Here, we determine mycobacterial MsRv1273c/72c to be an isoniazid efflux pump and determine several structures by cryo-electron microscopy showing specific asymmetrical features including an N-terminal extending loop and a periplasmic helical hairpin only found in MsRv1272c. Thus, MsRv1273c should have a degenerate site impaired for ATPase activity while MsRv1272c has a functional consensus site with the classic enzymatic motifs. Confirmation that this is correct was achieved by mutating both E553Q and D497N, creating the double mutant, which has little activity. Together, these results indicate that the consensus site of MsRv1273c/72c is functional with normal ATPase activity while its degenerate site exhibits very low activity. Thus, MsRv1273c/72c is a drug efflux pump for isoniazid, but not ethambutol.

Using single-particle 3D reconstruction, the cryo-EM structure of MsRv1273c/72c was determined at 3.1 Å resolution in the IFapo state. The central cavity is located between the two TMDs and it opens towards the cytoplasm. The two NBDs are separate at both NBSs. However, interactions are maintained between the two NBDs at their C-terminal helices. In the IFapo structure, the NBDs are separated both at consensus and degenerate sites by 8.4 Å and 10.7 Å, respectively. The N-terminal extending loop (includes residues 1-16, but only 10-16 are observed in the IFapo structure) of MsRv1272c wraps around TM6 by forming a right angle with the elbow helix (EH) and then interacts with the sidechain of Trp246 in TM4, which is conserved among the mycobacterial Rv1272c homologs. For example, the region containing a part of the D-loop, a part of the Walker B motif and the connecting residues (554AT555), which we assigned as the D-WalkerB loop (552DEATSSVD559), adopts a classical S-shaped conformation when the NBD binds nucleotide. However, the loop is adjusted to form an L-shaped conformation in the IFapo state. In this state, the catalytic residue, Glu553, points in the opposite direction to the consensus NBS. Thus, the consensus NBS is distorted in the IFapo state.

> SYFQSNMLWALLRQYVRPYRWLLAVVAVLQVISNMASLYLPTVNAAIIDDGVAKGDTARIVELGAVMLGVTALQVVCAVGAVFFGARAATGFGHDLRAAVFTHVTTFSAEEAGRFGAASLLTRTTNDVGHIQQLVQLTVTMLITAPIMSIGGIFMALHQDAGLSWLLLVSVPVLGLANYWIIRHLMPVFTRMQSLIDGINRVLRDQLSGIRVIRAFAREPLERVRFAEANQTLSDSALEAGRWQALMLPVTTLVINVSSVALIWFGGLRIDAGQMQVGSLIAFLAYFMQILMAVLMATFMLVIFPRAAVCADRIGEVLSTQTAITNPADPVRPAAIAGDIGVHDATFCYPGADRPVLQDVSFTVPRGTTTAVVGSTGSGKSTLISLICRLYDVTSGSLRIDGVDVRDLDIEQLWSAIGLVPQRGYLFSGTVAENLRYGRADATDDEMWEALRVAAAADFVRAHPQGLDMPVAQGGINFSGGQRQRLAIARAVIRRPAIYLFDDAFSALDVHTDARVRDALREVAADATVVIVSQRISTVIEADQVVVIDDGRVVGIGTHDTLLADCPIYAEFAESQALTAGEPR;> MRRGALPQAPLERTRDFKGSAIRLARRLLPQRALTLAVILLGVGGIAIGVIGPRILGHATDLLFNGVIGRELPAGLTKEQAVEAARARGDGTFADLLSGMDIVPGQGVDFGAVGRTLALALGLYLVAALLVWVQARLLNVTVQRTMVALRAEVQEKIHRLPLSYFDSRQRGEVLSRVTNDVDNIQNSVSMTISQLLTSVLTVFAVLVMMLTISPLLTLFTVVTVPASLWVTRWITRRSQPLFVAQWRNTGRLAAHLEETYSGFTIVKTFGHREAAAGKFAELNSETQQSSFGAQFFSGLVSPATMFIGNLSYVAVAVVGGLQVATGQITLGSIQAFIQYVRQFNQPLTQVAGMYNTLQSGIASAERVFDLLDTEEESADSPRRADVRTGRVEFEHVSFSYVPGTPVIEDLSLVAEPGSTVAIVGPTGAGKTTLVNLLMRFYDVDSGRITIDGVDIASVSRESLRASIGMVLQDTWLFAGTIYDNIAYGRPDADEDEVIEAATAAYVDRFVHTLPNGYDTRVDDDGGAISAGEKQLITIARAVLARPKLLVLDEATSSVDTRTELLIAHAMAELRRDRTSFIIAHRLSTIRDADLILVMDSGRIIERGTHEELLARHGRYWEMTRVHLGGIKAFHHHHHHHHHH> GPLGSPEFDCHLSDMLQQLHSVN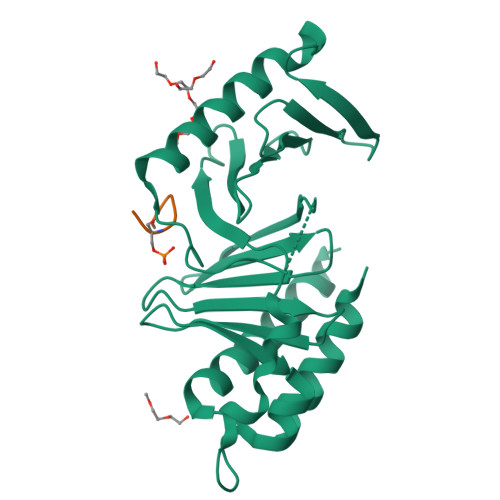ASKPSERGLVRQEEAEDPACIPIFWVSKWVDYSDKYGLGYQLCDNSVGVLFNDSTRLILYNDGDSLQYIERDGTESYLTVSSHPNSLMKKITLLKYFRNYMSEHLLKAGANITPREGDELARLPYLRTWFRTRSAIILHLSNGSVQINFFQDHTKLILCPLMAAVTYIDEKRDFRTYRLSLLEEYGCCKELASRLRYARTMVDKLLSSR;> XFMPPPMSSMX>MIGKRFFQTTSKKIAFAFDIDGVLFRGKKPIAGASDALKLLNRNKIPYILLTNGGGFSERARTEFISSKLDVDVSPLQIIQSHTPYKSLVNKYSRILAVGTPSVRGVAEGYGFQDVVHQTDIVRYNRDIAPFSGLSDEQVMEYSRDIPDLTTKKFDAVLVFNDPHDWAADIQIISDAINSENGMLNTLRNEKSGKPSIPIYFSNQDLLWANPYKLNRFGQGAFRLLVRRLYLELNGEPLQDYT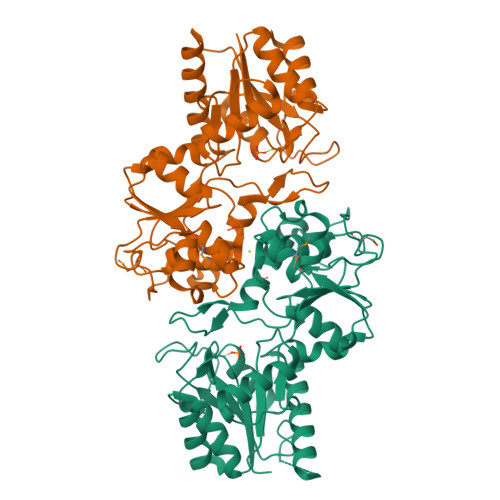LGKPTKLTYDFAHHVLIDWEKRLSGKIGQSVKQKLPLLGTKPSTSPFHAVFMVGDNPASDIIGAQNYGWNSCLVKTGVYNEGDDLKECKPTLIVNDVFDAVTKTLEKYA[2x]> GSHMASSCAVQVKLELGHRAQVRKKPTVEGFTHDWMVFVRGPEHSNIQHFVEKVVFHLHESFPRPKRVCKDPPYKVEESGWAGFILPIEVYFKNKEEPR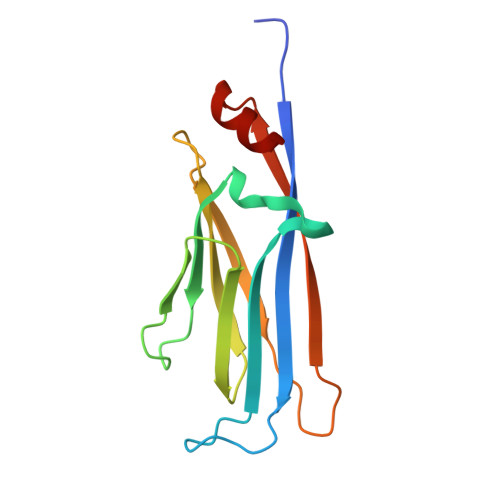KVRFDYDLFLHLEGHPPVNHLRCEKLTFNNPTEDFRRKLLKA2-(PHOSPHONOOXY)BUTANOIC ACID | C4 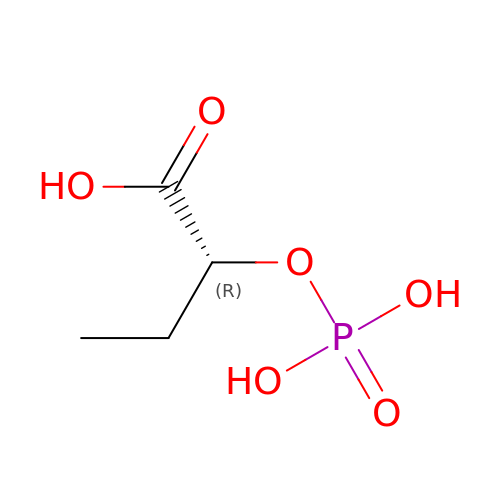H9 O6 P | OETAGSCBSKODFW-GSVOUGTGSA-N>[2x]DAVIP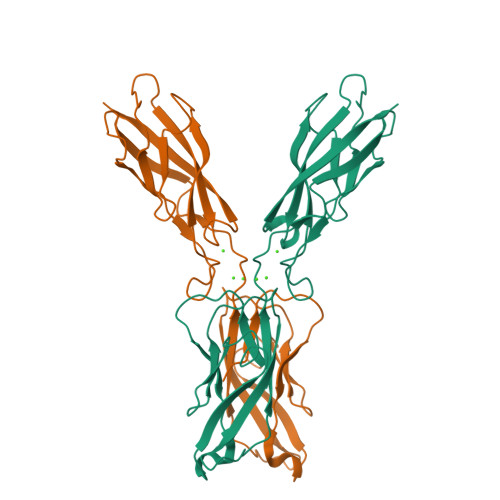PISCPENEKGEFPKNLVQIKSNRDKETKVFYSITGQGADKPPVGVFIIERETGWLKVTQPLDREAIAKYILYSHAVSSNGEAVEDPMEIVITVTDQNDNRPEFTQEVFEGSVAEGAVPGTSVMKVSATDADDDVNTYNAAIAYTIVSQDPELPHKNMFTVNRDTGVISVLTSGLDRESYPTYTLVVQAADLQGEGLSTTAKAVITVKD> MRTYSSLLEEFATELGLEEIETNELGHGAVTIDKIWVVHLAPINEKELVAFMRAGILTGQSQLYDILRKNLFSPLSGVIRCALDKDDHWLLWSQLNINDT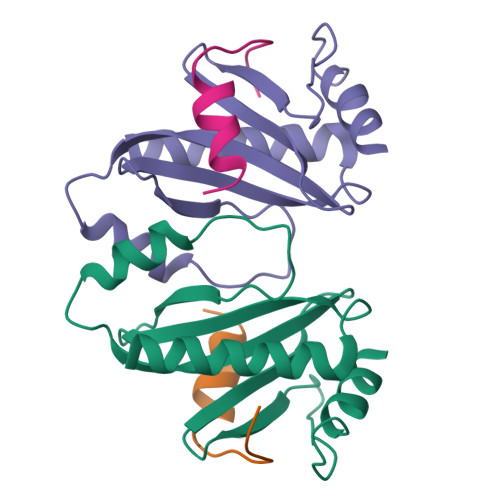SGTQLASVLTSLVDKAVTLSCEPTMKKEEDDHRPSSSH;> MTLQQVSTQAITSDERRFAYAVLEHAKNTILNRQDVAKLLPRASNFELSQHHHHHH>MFPDLKGKRVLITGSSQGIGLATARLFARAGAKVGLHGRKAPANIDETIASMRADGGDAAFFAADLATSEACQQLVDEFVAKFGGIDVLINNAGGLVGRKPLPEIDDTFYDAVMDANIRSVVMTTKFALPHLAAAAKASGQTSAVISTGSIA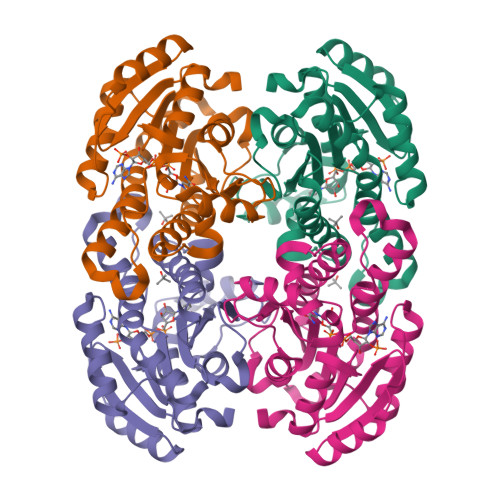GHTGGGPGAGLYGAAKAFLHNVHKNWVDFHTKDGVRFNIVSPGTVDTAFHADKTQDVRDRISNGIPMGRFGTAEEMAPAFLFFASHLASGYITGQVLDINGGQYKH[4x]>DQDEGVSTEPTQDGPAELPEDEECVFPFVYRNRKHFDCTVHGS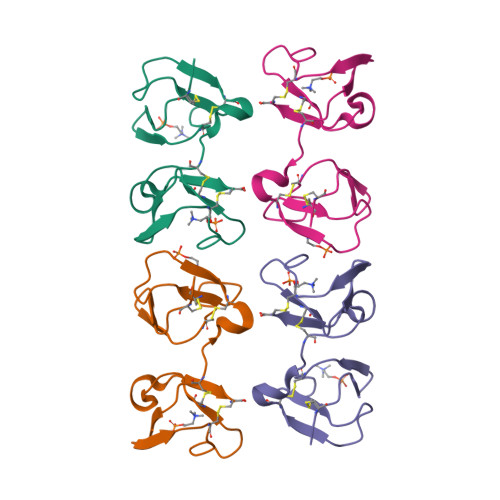LFPWCSLDADYVGRWKYCAQRDYAKCVFPFIYGGKKYETCTKIGSMWMSWCSLSPNYDKDRAWKYC[2x]> XHLTIHTWPEYGYAAIDLFTCGEDVDPWKAFEHLKKALKAKRVHVV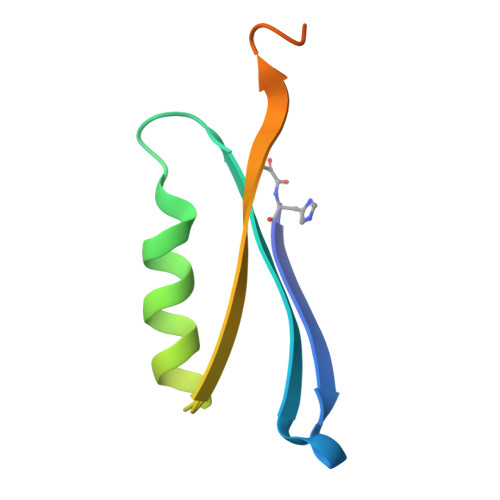EHERGRYDEIGIPEDSPHKAAV> MLKRKQSSRVEAQPVTDFGPDESLSDNADILWINKPWVHSLLRICAIISVISVCMNTPMTFEHYPPLQYVTFTLDTLLMFLYTAEMIAKMHIRGIVKGDSSYVKDRWCVFDGFMVFCLWVSLVLQVFEIADIVDQMSPWGMLRIPRPLIMIRAFRIYFRFELPRTRITNILKRSGEQIWSVSIFLLFFLLLYGILGVQMFGTFTYHCVVNDTKPGNVTWNSLAIPDTHCSPELEEGYQCPPGFKCMDLEDLGLSRQELGYSGFNEIGTSIFTVYEASSQEGWVFLMYRAIDSFPRWRSYFYFITLIFFLAWLVKNVFIAVIIETFAEIRVQFQQMWGTRSSTTSTATTQMFHEDAAGGWQLVAVDVNKPQGRAPACLQKMMRSSVFHMFILSMVTVDVIVAASNYYKGENFRRQYDEFYLAEVAFTVLFDLEALLKIWCLGFTGYISSSLHKFELLLVIGTTLHVYPDLYHSQFTYFQVLRVVRLIKISPALEDFVYKIFGPGKKLGSLVVFTASLLIVMSAISLQMFCFVEELDRFTTFPRAFMSMFQILTQEGWVDVMDQTLNAVGHMWAPLVAIYFILYHLFATLILLSLFV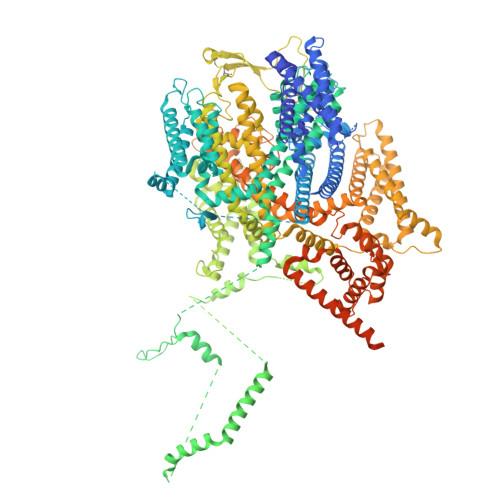AVILDNLELDEDLKKLKQLKQSEANADTKEKLPLRLRIFEKFPNRPQMVKISKLPSDFTVPKIRESFMKQFIDRQQQDTCCLFRILPSTSSSSCDNPKRPTVEDNKYIDQKLRKSVFSIRARNLLEKETAVTKILRACTRQRMLSGSFEGQPAKERSILSVQHHIRQERRSLRHGSNSQRISRGKSLETLTQDHSNTVRYRNAQREDSEIKMIQEKKEQAEMKRKVQEEELRENHPYFDKPLFIVGREHRFRNFCRVVVRARFNASKTDPVTGAVKNTKYHQLYDLLGLVTYLDWVMITVTICSCISMMFESPFRRVMHAPTLQIAEYVFVIFMSIELNLKIMADGLFFTPTAVIRDFGGVMDIFIYLVSLIFLCWMPQNVPAESGAQLLMVLRCLRPLRIFKLVPQMRKVVRELFSGFKEIFLVSILLLTLMLVFASFGVQLFAGKLAKCNDPNIIRREDCNGIFRINVSVSKNLNLKLRPGEKKPGFWVPRVWANPRNFNFDNVGNAMLALFEVLSLKGWVEVRDVIIHRVGPIHGIYIHVFVFLGCMIGLTLFVGVVIANFNENKGTALLTVDQRRWEDLKSRLKIAQPLHLPPRPDNDGFRAKMYDITQHPFFKRTIALLVLAQSVLLSVKWDVEDPVTVPLATMSVVFTFIFVLEVTMKIIAMSPAGFWQSRRNRYDLLVTSLGVVWVVLHFALLNAYTYMMGACVIVFRFFSICGKHVTLKMLLLTVVVSMYKSFFIIVGMFLLLLCYAFAGVVLFGTVKYGENINRHANFSSAGKAITVLFRIVTGEDWNKIMHDCMVQPPFCTPDEFTYWATDCGNYAGALMYFCSFYVIIAYIMLNLLVAIIVENFSLFYSTEEDQLLSYNDLRHFQIIWNMVDDKREGVIPTFRVKFLLRLLRGRLEVDLDKDKLLFKHMCYEMERLHNGGDVTFHDVLSMLSYRSVDIRKSLQLEELLAREQLEYTIEEEVAKQTIRMWLKKCLKRIRAKQQQSCSIIHSLRESQQQELSRFLNPPSIETTQPSEDTNANSQDHNTQPESSSQQQLLSPTLSDRGGSRQDAADTGKPQRKIGQWRLPSAPKPISHSVSSVNLRFGGRTTMKSVVCKMNPMPDTASCGSEVKKWWTRQLTVESDESGDDLLDI> XFSPAA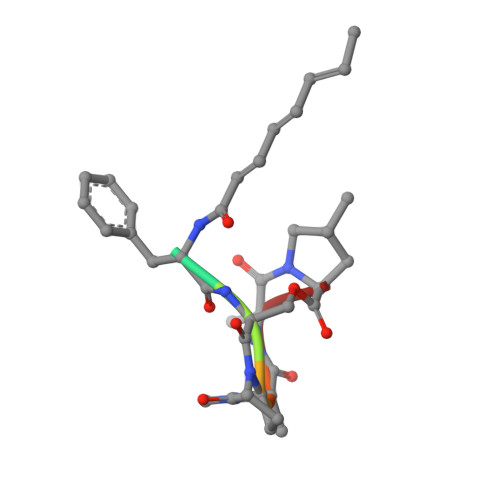P> MAPLENNYNESLNKSKDAIDDKTWSKLFPSIVSDPDRSSNFMIRAIYVVFSAVLRQRNILEKEYFSKNYITENLSCMTLSFKNLRAHQIAQLLRAAGDATKDGFLKEISLVVTEHDGDVEAIEVFSMKFIYFENGGVVARLSTDNNDQEDPHFAE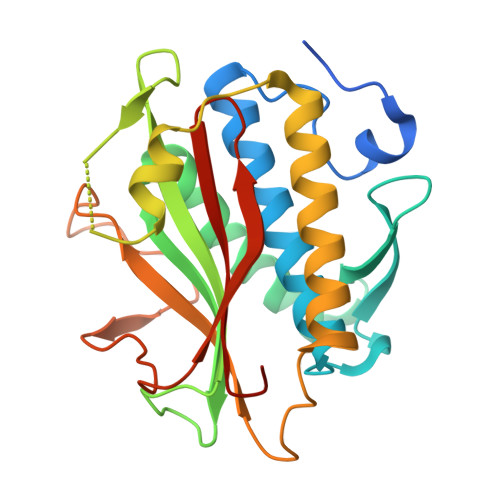LAQLRYEGAESVRDQMVTIVRSVQFLCTKVLEPLPAEFTANFRLKYTNDAPSNFRIDGFDDSSTFYTLPDGIQSVTIGHLRPGHHAAHMQCWSKSMSD>[8x]MKVNGVEVEETFAEAFDIKIARVLITGYDYYWAWVAANEATGFGTSVIMCPAEAGIEIKA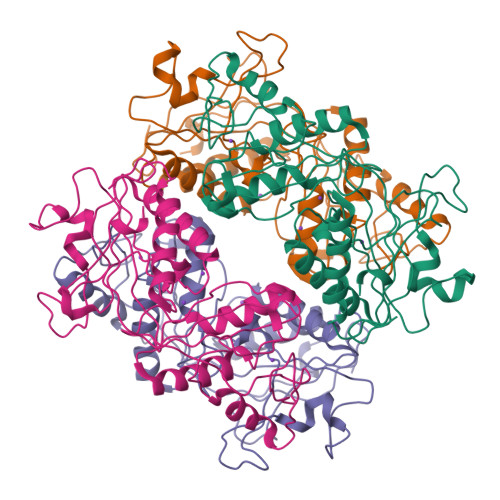KPSETPDGRPGYYIQICHMSKKGLEEQLLARLGQCVLTAPTTAVFNGLPDAEEKDDTGFKLKFFADGYQKEVEVGGRKCWAVPMMEGDFIIENDIGYTNGIAGGNFFIMAETQPSALAAAKAAVDAISDVEGVITPFPGGIVASGSKVGANKYKFLKASTNEKFAPSIRDQVEGTQIPAGVKAVYEIVINGLNADAIKEATRVGILAATKIPGVVKITAGNYGGKLGKHIINLNELF N-[(9S)-6-oxaspiro[4.5]decan-9-yl]methanesulfonamide | C10 H19 N O3 S | 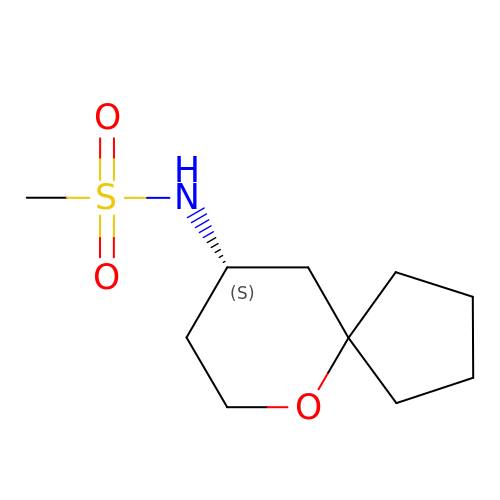FKSXOIFBVQFQLW-UHFFFAOYSA-N>AFYKREMFDPAEKYKMDHRRRGIALIFNHERFFWHLTLPERRGTCADRDNLTRRFSDLGFEVKCFNDLKAEELLLKIHEVSTVSHADADCFVCVFLSHGEGNHIYAYDAKIEIQTLTGLFKGDKCHSLVGKPKIFIIQACRGNQHDVPVIPLDVVDNQTEKLDTNITEVDAASVYTLPAGADFLMCYSVAEGYYSHRETVNGSWYIQDLCEMLGKYGSSLEFTELLTLVNRKVSQRRVDFCKDPSAIGKKQVPCFASMLTKKLHFFPKSNLEHHHHHH[2x];>[2x]XVE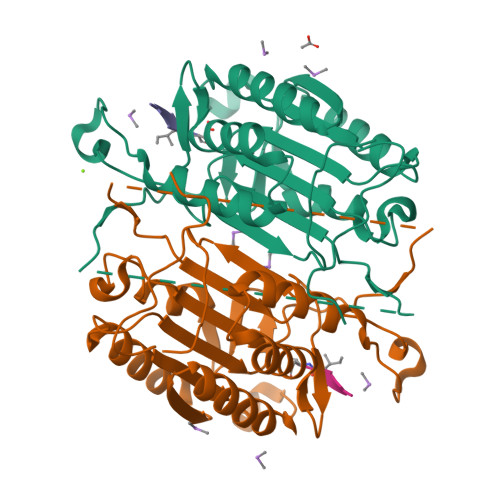ID> SNAMLLGVNIDHIAVLRQARMVNDPDLLEAAFIVARHGDQITLHVREDRRHAQDFDLENIIKFCKSPVNLECALNDEILNLALKLKPHRVTLVPEKREELTTEGGLCLNHAKL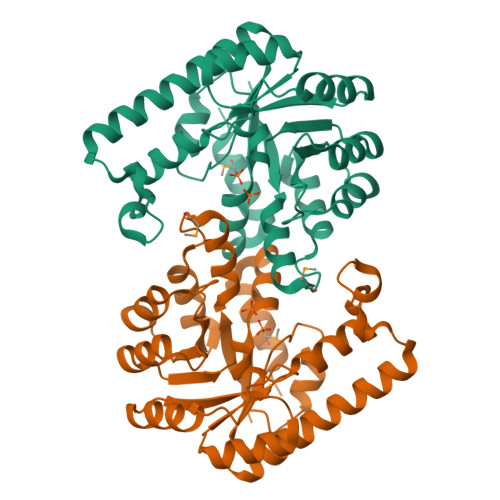KQSIEKLQNANIEVSLFINPSLEDIEKSKILKAQFIELHTGHYANLHNALFSNISHTAFALKELDQDKKTLQAQFEKELQNLELCAKKGLELGLKVAAGHGLNYKNVKPVVKIKEICELNIGQSIVARSVFTGLQNAILEMKELIKR> GPLG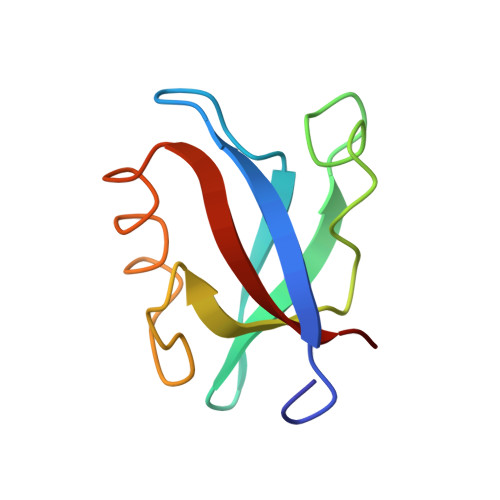SKIVRIEKARDIPLGATVRNEMDSVIISRIVKGGAAEKSGLLHEGDEVLEINGIEIRGKDVNEVFDLLSDMHGTLTFVLIPSQ PYRIDINE-2-CARBOXYLIC ACID | C6 H5 N O2 | 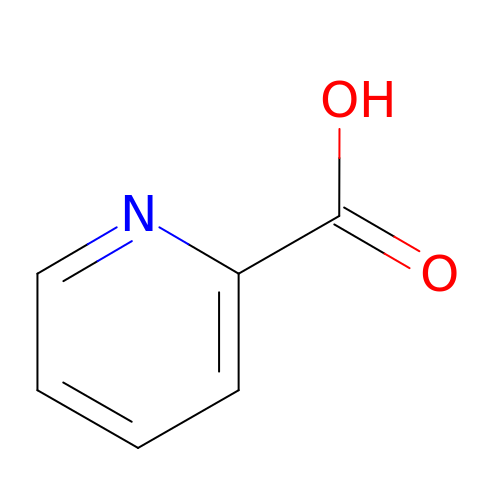SIOXPEMLGUPBBT-UHFFFAOYSA-N>MINVSDLTQKLPEGSNAGVIAKNINQNQIIADYNGSTFMLPASTQKVFTAVAAKLALGDQFQFETALLSNGKIQNGNLDGNLIVSFTGDPDLTRGQLYSLLAELKKQGIKKINGDLVLDTSVFSSHDRGLGWIWNDLTMCFNSPPAAANIDNNCFYAELDANKNPGEIVKINVPAQFPIQVFGQVYVADSNEAPYCQLDVVVHDNNRYQVKGCLARQYKPFGLSFAVQNTDAYAAAIIQRQLRKLGIEFNGKVLLPQKPQQGQLL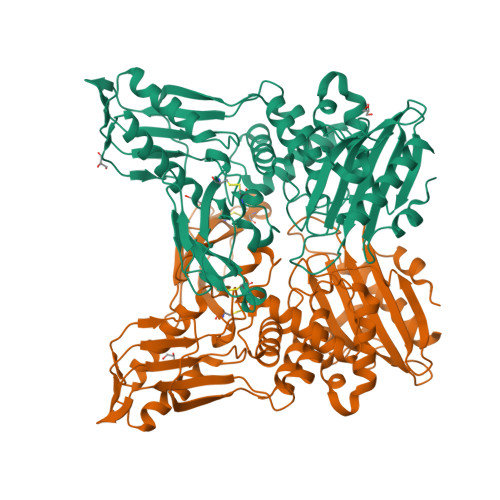AKHLSKPLPDLLKKMMKKSDNQIADSLFRAVAFNYYKRPASFQLGTLAVKSILQKQGIRFGNSILADGSGLSRHNLVAPKTMLSVLEYIAKNEDKLHLMETFPIAGVDGTISGRGGLISPPLVKNVIAKTGSLKGVYNLAGFMTNARGEKVAFVQFINGYSTGDLESKTKRAPLVQFERNLYNELYKY[2x]> QKTGTAEMSSILEERILGADTSVDLEETGRVLSIGDGIARVHGLRNVQAEEMVEFSSGLKGMSLNLEPDNVGVVVFGNDKLIKEGDIVKRTGAIVDVPVGDELLGRVVDALGNAIDGKGPVGSKIRRRVGLKAPGIIPRISVREPMQTGIKAVDSLVPIGRGQRELIIGDRQTGKTSIAIDTIINQKRFNDGTDEKKKLYCIYVAIGQKRSTVAQLVKRLTDADAMKYTIVVSATASDAAPLQYLAPYSGCSMGEYFRDNGKHALIIYDDLSKQAVAYRQMSLLLRRPPGREAYPGDVFYLHSRLLERAAKMNDSFGGGSLTALPVIETQAGDVSAYIPTNVISITDGQIFLETELFYKGIRPAINVGLSVSRVGSAAQTRAMKQVAGTMKLELAQYREVAAFAQFGSDLDAATQQLLSRGVRLTELLKQGQYSPMAIEEQVAVIYAGVRGYLDKLEPSKITKFESAFLSHVVSQHQSLLGNIRTDGKISEQSDAKLKEIVTNFLAGFEP;> SAAPKAGTATGQIVAVIGAVVDVQFDEGLPPILNALEVQGRESRLVLEVAQHLGESTVRTIAMDGTEGLVRGQKVLDSGAPIKIPVGPETLGRIMNVIGEPIDERGPIKTKQFAPIHAEAPEFIEMSVEQEILVTGIKVVDLLAPYAKGGKIGLFGGAGVGKTVLIMELINNVAKAHGGYSVFAGVGERTREGNDLYHEMIESGVINLKDATSKVALVYGQMNEPPGARARVALTGLTVAEYFRDQEGQDVLLFIDNIFRFTQAGSEVSALLGRIPSAVGYQPTLATDMGTMQERITTTKKGSITSVQAIYVPADDLTDPAPATTFAHLDATTVLSRAIAELGIYPAVDPLDSTSRIMDPNIVGSEHYDVARGVQKILQDYKSLQDIIAILGMDELSEEDKLTVSRARKIQRFLSQPFQVAEVFTGHMGKLVPLKETIKGFQQILAGDYDHLPEQAFYMVGPIEEAVAKADKLAEEHGS;> RDITRRLKSIKNIQKITKSMKMVAAAKYARAERELKPARVYGTGSLALYEKAEIKGPEDKKKHLIIGVSSDRGLCGAIHSSVAKQMK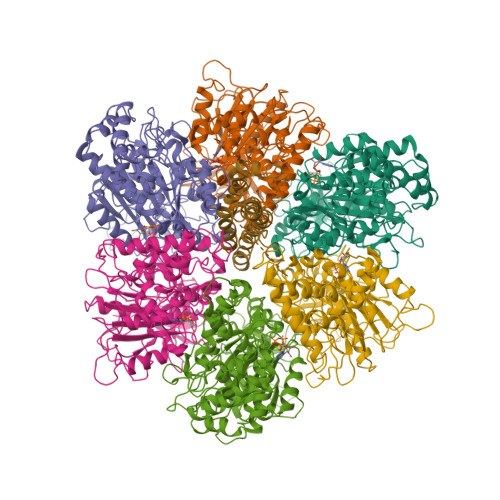NDMAALTAAGKEVMIVGIGEKIKSILYRTHSDQFLVSFKDVGRKPPTFGDASVIALELLNSGYEFDEGSIIFNQFKSVISYKTEEKPIFSFSTVVAAENMSIYDDIDADVLQNYQEYNLANIIYYSLKESTTSEQSARMTAMDNASKNASDMIDKLTLTFNRTRQAVITKELIEIISGAAALD> STSLPTSNEYQNEKLANELKSLLDELNVNELATGSLNTYYKRTIKISGQKAMYALKSK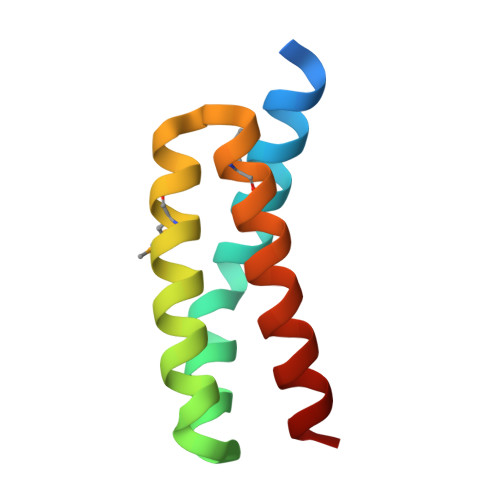DFKKMSEAKYQLQKIYNEIDEALK> GAMLVRETGHAPFRAQALALDADAALSEAFPAILGNCLEHIQRNEVAVIEGHDPETLHQMRVGVRRLRSALKLFDAVAPCPPALQDDISWLGTELGAARDWDVLLASTLPRIDGAPAGANGLLELNALVQKIAQAKRHAAAQALLSPRYTRLMLTLGAWMLETAPLLDGSAAHFSRQIMQH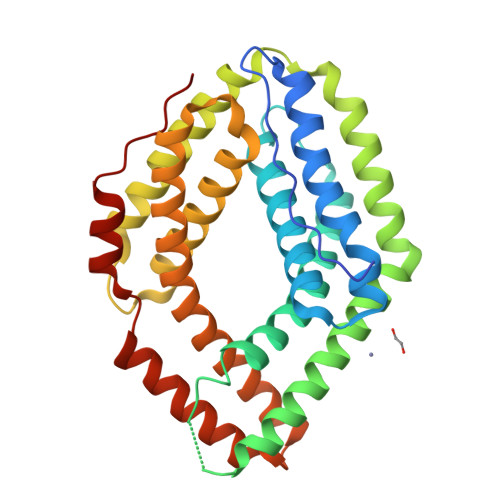LHKSLLKRAARMQDDDAASAHRTRIATKRGRYALEFFHGLYRSKSTRAYLKALAATQEELGRHNDLVVAGRLLQELAQQQPQAAEAVQFARGYLLAQQAMRPADLDAIRAGLHALRAPQLRH>[6x]AINLIDLLHDGFYLIFLIRNQYVPADPQRFREKILDLLNRFEQQAKKLQFSADDIHDAKYAFCALIDETIVTQQDPSYFNLQN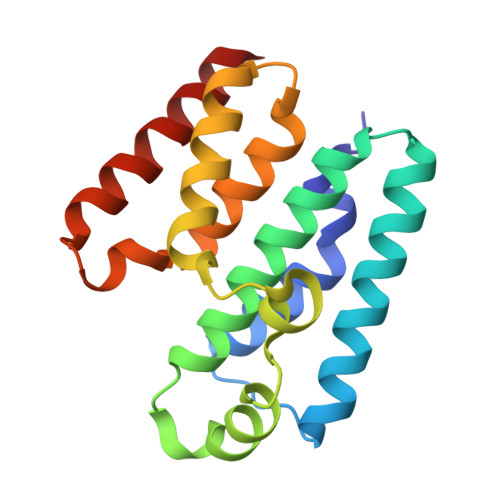SWLISPLQLSLFGSQLAGYQFFEILEQLRSRGKERLAALEVFHYCLLLGFQGKYRIESIESLNHLVARVGDEIDYLKG>[2x]RFLKVKNWETDVVLTDTLHLKSTLETGCTEHICMGSIMLPSQHTRKPEDVRTKDQLFPLAKEFLDQYYSSIKRFGSKAHMDRLEEVNKEIESTSTYQLKDTELIYGAKHAWRNASRCVGRIQWSKLQVFDARDCTTAHGMFNYICNHVKYATNKGNLRSAITIFPQRTDGKHDFRVWNSQLIR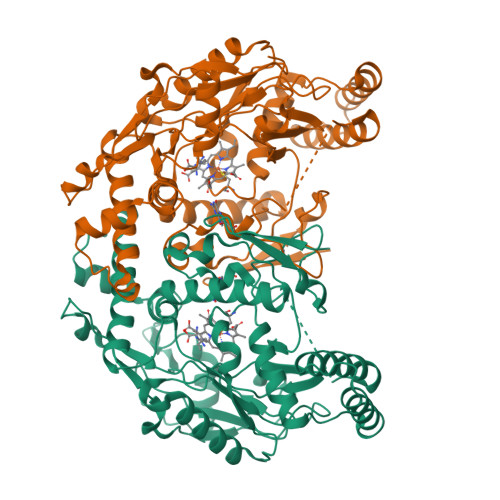YAGYKQPDGSTLGDPANVQFTEICIQQGWKAPRGRFDVLPLLLQANGNDPELFQIPPELVLEVPIRHPKFDWFKDLGLKWYGLPAVSNMLLEIGGLEFSACPFSGWYMGTEIGVRDYCDNSRYNILEEVAKKMDLDMRKTSSLWKDQALVEINIAVLYSFQSDKVTIVDHHSATESFIKHMENEYRCRGGCPADWVWIVPPMSGSITPVFHQEMLNYRLTPSFEYQPDPWNTHVWKG> MSNWVMQEENKQGNLTPLFEELLQQCPPGGQNKTAHMVSAYQLAQGNWMPTSCHVFMGTISARRTKTHPYEAYVKLRELVEEHKMKTLCPGSSLGKHNDWIIGKIKYQGNLRTKHMLNPGKVAEQLCREGHRHNVYNKTIGS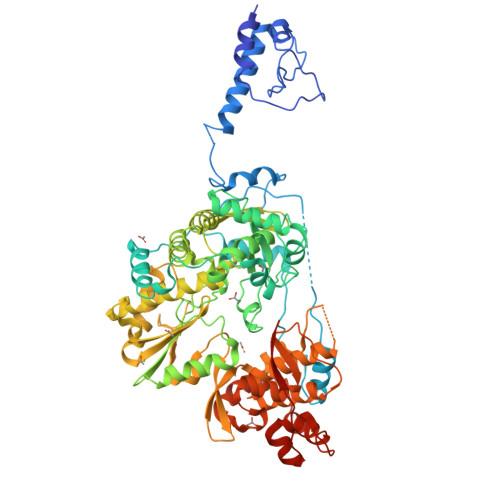VMTATGIRLEKLPVVRAQTDTTNFHQAIRDKIDKEENLQTPGLHKKLMEVFNALKRPELESSYDAVEWEELERGINRKGAAGFFERKNIGEILDSEKNKVEEIIDNLKKGRNIKYYETAIPKNEKRDVNDDWTAGDFVDEKKPRVIQYPEAKTRLAITKVMYKWVKQKPVVIPGYEGKTPLFQIFDKVKKEWDQFQNPVAVSFDTKAWDTQVTTKDLELIKDIQKYYFKKKWHKFIDTLTMHMTEVPVICADGEVYIRKGQRGSGQPDTSAGNSMLNVLTMVYAFCEATGVPYKSFDRVAKIHVCGDDGFLITERALGEKFASKGVQILAAAGKPQKITEGDKMKVAYQFDDIEFCSHTPIQVRWSDNTSSYMPGRNTTTILAKMATRLDSSGERGTIAYEKAVAFSFLLMYSWNPLIRRICLLVLSTELQVKPGKSTTYYYEGDPISAYKEVIGHNLFDLKRTSFEKLAKLNLSMSVLGAWTRHTSKRLLQDCVNMGVKEGNWLVNADRLVSSKTGNRYIPGEGHTLQGRGSSSHHHHHH>[2x]MASMTGGQQMGRGSEFAKAPEQTVTEPVGSYARAERPQDFEGFVWRLDNDGKEALPRNFRTSADALRAPEKKFHLDAAYVPS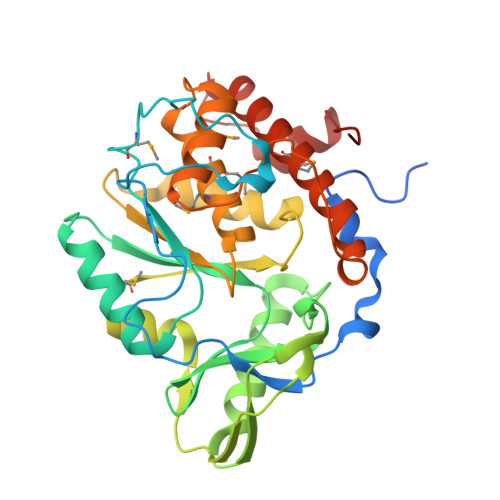REGMDALHISGSSAFTPAQLKNVAAKLREKTAGPIYDVDLRQESHGYLDGIPVSWYGERDWANLGKSQHEALADERHRLHAALHKTVYIAPLGKHKLPEGGEVRRVQKVQTEQEVAEAAGMRYFRIAATDHVWPTPENIDRFLAFYRTLPQDAWLHFHCEAGVGRTTAFMVMTDMLKNPSVSLKDILYRQHEIGGFYYGEFPIKTKDKDSWKTKYYREKIVMIEQFYRYVQENRADGYQTPWSVWLKSHPAKALE> GSVDQNIPRGAVLHSEPLTVMVLTATDPFEYESPEHEVKNMLHATVATVSQYFHVKVFNINLKEKFTKKNFIIISNYFESKGILEINETSSVLEAAPDQMIEVPNSIIRNANASPKICDIQKGTSGAVFYGVFTLHKKTVNRKNTIYEIKDGSGSIEVVGSGKWHNINC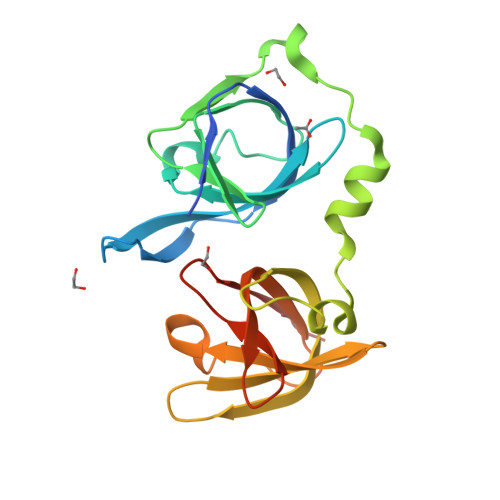KEGDKLHLFCFHLKTIDRQPKLVCGEHSFIKISKRGNAAAS>[7x]MEQTQKLKLNLQHFASNNVKPQVFNPDNVMMHEKKDGTLMNEFTTPILQEVMENSKIMQLGKYEPMEGTEKKFTFWADKPGAYWVGEGQKIETSKAT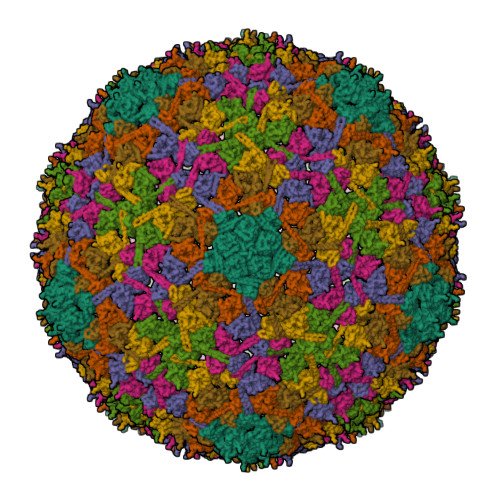WVNATMRAFKLGVILPVTKEFLNYTYSQFFEEMKPMIAEAFYKKFDEAGILNQGNNPFGKSIAQSIEKTNKVIKGDFTQDNIIDLEALLEDDELEANAFISKTQNRSLLRKIVDPETKERIYDRNSDSLDGLPVVNLKSSNLKRGELITGDFDKLIYGIPQLIEYKIDETAQLSTVKNEDGTPVNLFEQDMVALRATMHVALHIADDKAFAKLVPADKRTDSVPGEV> YTPSSASTVSVGSS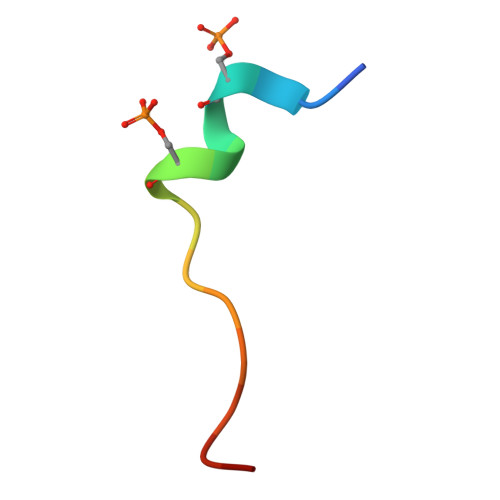ET> SSDSEDVVSPNCSNTVQEKTFNKDTVIIVSEPSEDEESQGLPTMARRNDDISELEDLSELEDLKDAKLQTLKELFPQRSDNDLLKLIESTSTMDGAIAAALLMFGDAGGGPR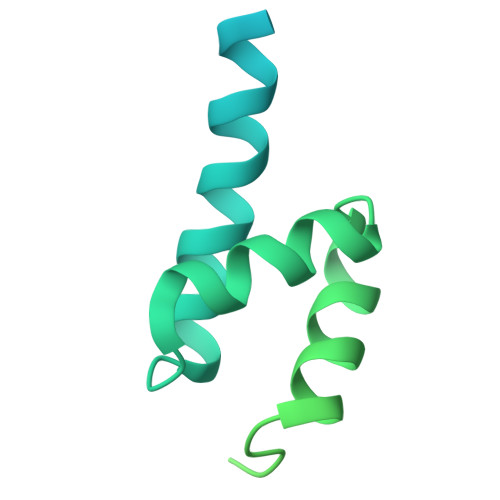KRKLSSSSEPYEEDEFNDDQSIKKTRLDHGEESNESAESSSNWEKQESIVLKLQKEFPNFDKQELREVLKEHEWMYTEALESLKVFAEDQDMQYVSQSEVPNGKEVSSRSQNYPKNATKTKLKQKFSMKAQNGFNKKRKKN>[6x]MKHHHHHHGSSGMQDQIDAKVIRRNPELTPGIFKKGIEITIDLEEMVCYHSGLTWKVKQLTNTLWSLAGDEHTVMEVI

We recently identified and characterized a fused toxin–antitoxin system called CapRelSJ46 that protects Escherichia coli against diverse phages. CapRelSJ46 contains an N-terminal toxin domain and a C-terminal antitoxin domain that normally binds and autoinhibits the N-terminal toxin. Activated CapRelSJ46 then pyrophosphorylates the 3′ end of transfer RNAs, which inhibits protein translation and restricts phage propagation. Here we discovered an additional protein trigger for CapRelSJ46 in the phage Bas11. This alternative trigger, Gp54Bas11, is a small protein of 66 amino acids with unknown function.

To gain better structural insight into the interaction between CapRelSJ46 and Gp54Bas11, we first solved a crystal structure of Gp54Bas11 to 2.3 Å resolution. This structure showed a small, six-stranded β-barrel with one prominent loop between β-strands β1 and β2; β-barrels with this topology are very rare in nature. The closest structural homologues of Gp54Bas11 are five-stranded β-barrel SH3 domains (DALI z-score of 3.8), with a 310 α-helix replacing the additional β-strand. Thus, the structure of Gp54Bas11 is significantly distinct from the AlphaFold-predicted structure of MCP from SECΦ27, with root mean square deviation (r.m.s.d.) greater than 14 Å. By contrast, A7 is disordered in the complex but is part of the β-barrel core in unbound Gp54Bas11. The A7V substitution may have stabilized the unbound β-barrel, which would also have prevented activation by preventing the unfolding of Gp54Bas11. We verified that the G24D variant was still properly folded because it had a circular dichroism spectrum comparable to the wild-type protein.> MRVLVTGGSGYIGSHTCVQLLQNGHDVIILDNLCNSKRSVLPVIERLGGKHPTFVEGDIRNEALMTEILHDHAIDTVIHFAGLKAVGESVQKPLEYYDNNVNGTLRLISAMRAANVKNFIFSSSATVYGDNPKIPYVESFPTGTPQSPYGKSKLMVEQILTDLQKAQPDWSIALLRYFNPVGAHPSGDMGEDPQGIPNNLMPYIAQVAVGRRDSLAIFGNDYPTEDGT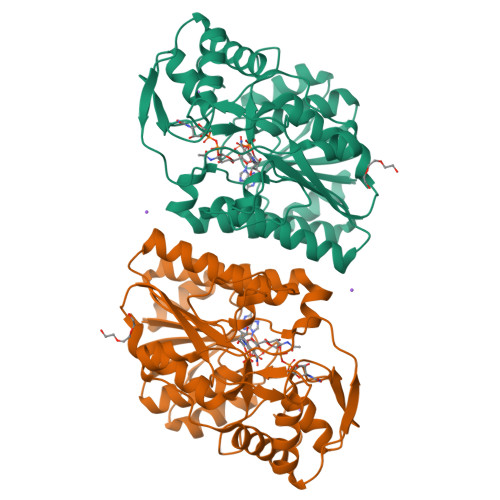GVRDYIHVMDLADGHVVAMEKLANKPGVHIYNLGAGVGNSVLDVVNAFSKACGKPVNYHFAPRREGDLPAYWADASKADRELNWRVTRTLDEMAQDTWHWQSRHPQGYPD> MKEKIFNELTRKMKRKEISAKIQREENKQILIRQRNNKKYIQSIQGIQQERKKGKLYLVEMATQNVEEMDTIQKMNYEATVNMGRQDLITREYTFYSDYEFIP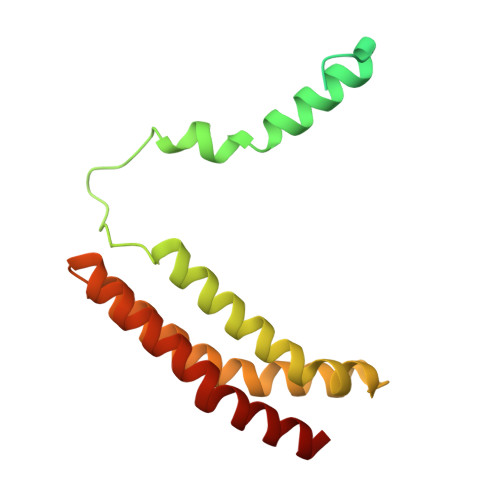IQEDRKQQMEDALNNLHKIIHPTVTQLKKKANVQEIQDRVFRKLQGWEGELNTCVFSAKNVRDSNFCADRFTNRINTEGVEFVKQILREY> MKPEIEQELSHTLLTELLAYQFASPVRWIETQDVFLKQHNTERIIEIGPSPTLAGMANRTIKAKYESYDAALSLQRQVLCYSKDAKEIYYKPDPADLAPKETPKQEESTPSAPAAATPTPAAAAAPTPAPAPASAGPVESIPDEPVKANLLIHVLVAQKLKKPLDAVPMTKAIKDLVNGKSTVQNEILGDLGKEFGSTPEKPEDTPLEELAEQFQDSFSGQLGKTSTSLIGRLMSSKMPGGFSITTARKYLESRFGLGAGRQDSVLLMALTNEPANRLGSEADAKTFFDGIAQKYASSAGISLSSGAGSGAGAANSGGAVVDSAALDALTAENKKLAKQQLEVLARYLQVDLNKGSAKSFIKEKEASAVLQKELDLWEAEHGEFYAKGIQPTFSALKSRTYDSYWNWARQDVLSMYFDIIFGKLTSVDRETINQCIQIMNRANPTLIKFMQYHIDHCPEYKGETYKLAKRLGQQLIDNCKQVLTEDPVYKDVSRITGPKTKVSAKGNIEYEETQKDSVRKFEQYVYEMAQGGAMTKVSQPTIQEDLARVYKAISKQASKDSKLELQRVYEDLLKVVESSKEIETEQLTKDILQAATVPTTPTEEVDDPCTPSSDDEIASLPDKTSIIQPVSSTIPSQTIPFLHIQKKTKDGWEYNKKLSSLYLDGLESAAINGLTFKDKYVLVTGAGAGSIGAEILQGLISGGAKVIVTTSRFSKKVTEYYQNMYARYGAAGSTLIVVPFNQGSKQDVDALVQYIYDEPKKGGLGWDLDAIIPFAAIPENGNGLDNIDSKSEFAHRIMLTNLLRLLGAVKSKKTTDTRPAQCILPLSPNHGTFGFDGLYSESKISLETLFNRWYSEDWGSKLTVCGAVIGWTRGTGLMSANNIIAEGIEKLGVRTFSQKEMAFNILGLLTPEIVQLCQEEPVMADLNGGLQFIDNLKDFTSKLRTDLLETADIRRAVSIESAIEQKVVNGDNVDANYSKVMVEPRANMKFDFPTLKSYDEIKQIAPELEGMLDLENVVVVTGFAEVGPWGNSRTRWEMEAYGEFSLEGAIEMAWIMGFIKYHNGNLKGKPYSGWVDAKTQTPIDEKDIKSKYEEEILEHSGIRLIEPELFNGYDPKKKQMIQEVVVQHDLEPFECSKETAEQYKHEHGEKCEIFEIEESGEYTVRILKGATLYVPKALRFDRLVAGQIPTGWDARTYGIPEDTISQVDPITLYVLVATVEALLSAGITDPYEFYKYVHVSEVGNCSGSGMGGVSALRGMFKDRYADKPVQNDILQESFINTMSAWVNMLLLSSSGP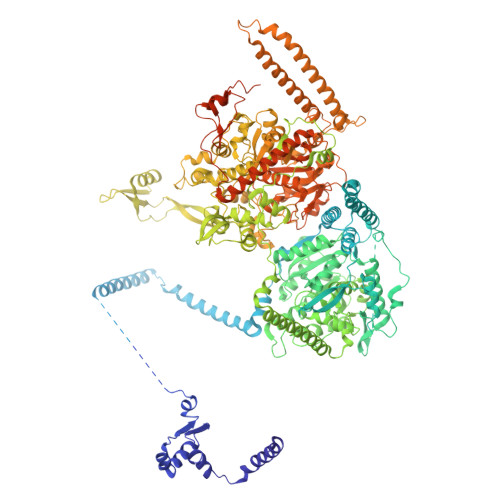IKTPVGACATAVESVDIGIETILSGKAKVVLVGGYDDFQEEGSYEFANMNATSNSIEEFKHGRTPKEMSRPTTTTRNGFMEAQGSGIQVIMTADLALKMGVPIHAVLAMTATATDKIGRSVPAPGKGILTTAREHHGNLKYPSPLLNIEYRKRQLNKRLEQIKSWEETELSYLQEEAELAKEEFGDEFSMHEFLKERTEEVYRESKRQVSDAKKQWGNSFYKSDPRIAPLRGALAAFNLTIDDIGVASFHGTSTVANDKNESATINNMMKHLGRSEGNPVFGVFQKYLTGHPKGAAGAWMLNGAIQILESGLVPGNRNADNVDKLLEQYEYVLYPSRSIQTDGIKAVSVTSFGFGQKGAQAVVVHPDYLFAVLDRSTYEEYATKVSARNKKTYRYMHNAITRNTMFVAKDKAPYSDELEQPVYLDPLARVEENKKKLVFSDKTIQSSQSYVGEVAQKTAKALSTLNKSSKGVGVDVELLSAINIDNETFIERNFTGNEVEYCLNTAHPQASFTGTWSAKEAVFKALGVESKGAGASLIDIEITRDVNGAPKVILHGEAKKAAAKAGVKNVNISISHDDFQATAVALSEF> LQPATAEAADSYKIVGYYPSWAAYGRNYNVADIDPTKVTHINYAFADICWNGIHGNPDPSGPNPVTWTCQNEKSQTINVPNGTIVLGDPWIDTGKTFAGDTWDQPIAGNINQLNKLKQTNPNLKTIISVGGWTWSNRFSDVAATAATREVFANSAVDFLRKYNFDGVDLDWEYPVSGGLDGNSKRPEDKQNYTLLLSKIREKLDAAGAVDGKKYLLTIASGAS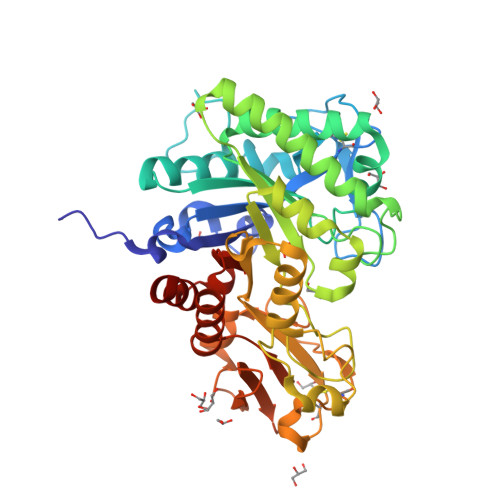ATYAANTELAKIAAIVDWINIMTYDFNGAWQKISAHNAPLNYDPAASAAGVPDANTFNVAAGAQGHLDAGVPAAKLVLGVPFYGRGWDGCAQAGNGQYQTCTGGSSVGTWEAGSFDFYDLEANYINKNGYTRYWNDTAKVPYLYNASNKRFISYDDAESVGYKTAYIKSKGLGGAMFWELSGDRNKTLQNKLKADL> ATTQIGEIVKTVANTVESEIKAELGVIPSLNAVETGATSNTEPEEAIQTRTVINMHGTAECLVENFLGRSALVCMRSFEYKNHSTSTSSIQKNFFIWTLNTRELVQIRRKMELFTYLRFDTEITIVPTLRLFSSSNVSFSGLPNLTLQAMYVPTGARKPSSQDSFEWQSACNPSVFFKINDPPARLTIPFMSINSAYANFYDGFAGFEKKATVLYGINPANTMGNLCLRVVNSYQPVQYTLTVRVYMKPKHIKAWAPRAPRTMPYTNILNNNYAGRSAAPNAPTAIVSHRSTIKTMPNDINLTTA;> SPSAEACGYSDRVLQLKLGNSSIVTQEAANICCAYGEWPTYLPDNEAVAIDKPTQPETSTDRFYTLKSKKWESNSTGWWWKLPDALNQIGMFGQNVQYHYLYRSGFLCHVQCNATKFHQGTLLIVAIPEHQIGKKGTGTSASFAEVMKGAEGGVFEQPYLLDDGTSLACALVYPHQWINLRTNNSATIVLPWMNSAPMDFALRHNNWTLAVIPVCPLAGGTGNTNTYVPITISIAPMCAEYNGLRNAITQ;> GVPTCLLPGSNQFLTTDDHSSAPAFPDFSPTPEMHIPGQVHSMLEIVQIESMMEINNVNDASGVERLRVQISAQSDMDQLLFNIPLDIQLEGPLRNTLLGNISRYYTHWSGSLEMTFMFCGSFMTTGKLIICYTPPGGSSPTDRMQAMLATHVVWDFGLQSSITIIIPWISGSHYRMFNTDAKAINANVGYVTCFMQTNLVAPVGAADQCYIVGMVAAKKDFNLRLMRDSPDIGQSAILPEQA;> GAQVSRQQTGTHENANVATGGSSITYNQINFYKDSYAASASKQDFSQDPSKFTEPVAEALKAGAPVLK

Enterovirus 70 (EV70) is a human pathogen belonging to the family Picornaviridae. EV70 is transmitted by eye secretions and causes acute hemorrhagic conjunctivitis, a serious eye disease. The capsid of EV70 is composed of the subunits VP1, VP2, VP3, and VP4. The major capsid proteins of EV70 are organized with pseudo-T=3 icosahedral symmetry, with VP1 subunits forming pentamers around 5-fold symmetry axes and VP2 and VP3 subunits forming heterohexamers at 3-fold axes of the capsid.

Here, we show that WIN51711 and pleconaril inhibit EV70 with 50% effective concentration (EC50) values of 0.26 μM and 0.45 μM, respectively. We found that the binding of the inhibitors increases the melting temperature (Tm) of EV70 from 48.9°C for the virion to 51.6°C and 50.6°C for particles treated with WIN51711 and pleconaril, respectively. Cryo-EM reconstructions of complexes of EV70 with WIN51711 and pleconaril were determined to resolutions of 2.74 Å and 2.31 Å, respectively. The binding of the inhibitors induced the expansion of the VP1 pocket, which required a 1-Å movement of residues Met112, Met192, and Met224 of VP1 away from the core of the subunit relative to the structure of the subunit in the native virion. Notably, the side chain of Met224, which partially blocked the pocket in the native particle, now adopts a conformation that allows the presence of the inhibitor without changing the position of the VP1 GH loop backbone, in contrast to EV-D68, where the presence of the inhibitor induces changes in the backbone. There are 26 residues of VP1 that interact with pleconaril or WIN51711. Most of the interactions between VP1 and the inhibitors are hydrophobic. Moreover, 4 hydrogen bonds connect pleconaril to VP1, providing specificity to the inhibitor-capsid interactions. The GH loop from VP1 of EV-D68 becomes disordered when pleconaril binds to the pocket; a similar loss of the structure of the loop was not observed for EV70. The structures of EV70, EV-D68, HRV14, and HRV16 in complex with pleconaril show that the isoxazole and trifluoromethyl ends of the molecule occupy equivalent spaces in the pockets of these viruses.>TPFIRPDMKAFLEAIAAMAGPTLAEMTLEEARASYVALHGMADRPARELAVIRNLSCPGPAGDIPLRLYDARESREAGPVITFYHGGGFVIGDLDTHHNLCTEIAALMDLPVVAVDYRLAPEHPFPAAIEDCEAATRWVASSPSELGRTASGVIPIGDAAGGNATIVVSQLLGAKPADVPVVLQVPIFPLASDAVGSASLEAFAEGFVLTKASIEFFDTAYKADRADPRGFPILGDHTAAPPTIVATASLD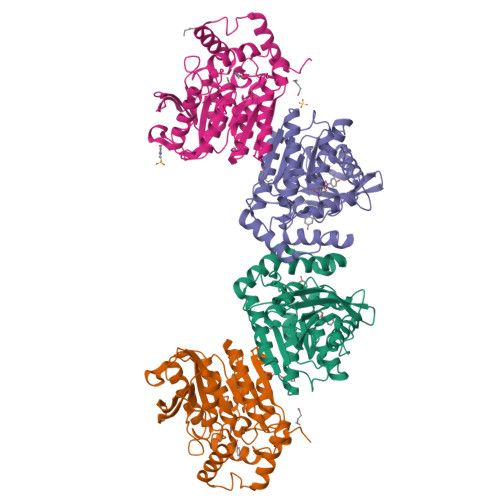PIRDSGRDYAKALVEAGRDVVYLEMEGVTHSFTNIRAAVPSTQGDLERIIAAMKMMLG[3x];> DTPFIRPDMKAFLEAIAAMAGPTLAEMTLEEARASYVALHGMADRPARELAVIRNLSCPGPAGDIPLRLYDARESREAGPVITFYHGGGFVIGDLDTHHNLCTEIAALMDLPVVAVDYRLAPEHPFPAAIEDCEAATRWVASSPSELGRTASGVIPIGDAAGGNATIVVSQLLGAKPADVPVVLQVPIFPLASDAVGSASLEAFAEGFVLTKASIEFFDTAYKADRADPRGFPILGDHTAAPPTIVATASLDPIRDSGRDYAKALVEAGRDVVYLEMEGVTHSFTNIRAAVPSTQGDLERIIAAMKMMLG>[2x]HNCFCIQEVVSGLRQPVGALHSGDGSQRLFILEKEGYVKILTPEGEIFKEPYLDIHKLVQSGIKGGDERGLLSLAFHPNYKKNGKLYVSYTTNQERWAIGPHDH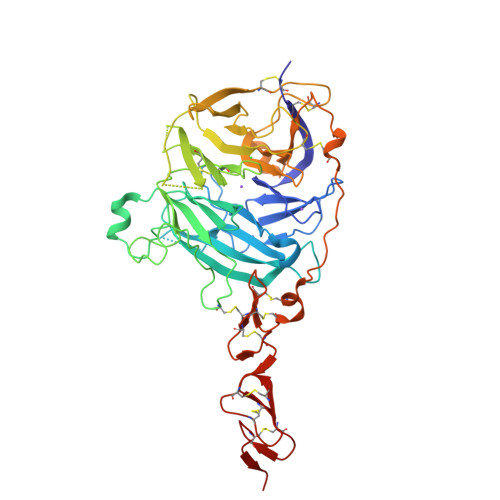ILRVVEYTVSRKNPHQVDLRTARVFLEVAELHRKHLGGQLLFGPDGFLYIILGDGMITLDDMEEMDGLSDFTGSVLRLDVDTDMCNVPYSIPRSNPHFNSTNQPPEVFAHGLHDPGRCAVDRHPTDININLTILCSDSNGKNRSSARILQIIKGKDYESEPSLLEFKPFSNGPLVGGFVYRGCQSERLYGSYVFGDRNGNFLTLQQSPVTKQWQEKPLCLGTSGSCRGYFSGHILGFGEDELGEVYILSSSKSMTQTHNGKLYKIVDPKRPLMPEECRATVQPAQTLTSECSRLCRNGYCTPTGKCCCSPGWEGDFCRTAKCEPACRHGGVCVRPNKCLCKKGYLGPQCEQVDR>MVALQIPSLAATVRQDFPILNQEINGHPLVYLDNAATSQKPRAVLEKLMHYYENDNANVHRGAHQLSVRATDA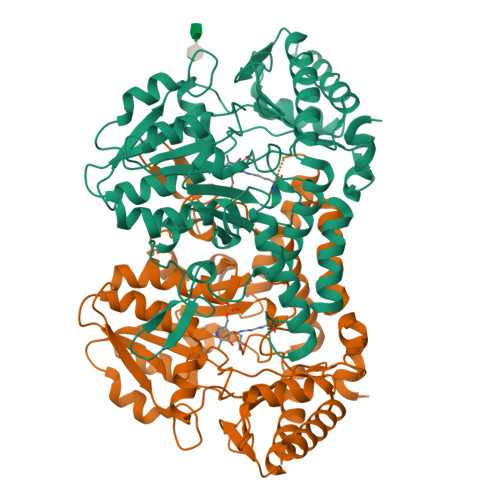YEAVRNKVAKFINARSPREIVYTRNATEAINLVAYSWGMNNLKAGDEIITTVMEHHSNLVPWQMVAAKTGAVLKFVQLDEQESFDLEHFKTLLSEKTKLVTVVHISNTLGCVNPAEEIAQLAHQAGAKVLVDACQSAPHYPLDVQLIDCDWLVASGHKMCAPTGIGFLYGKEEILEAMPPFFGGGEMIAEVFFDHFTTGELPHKFEAGTPAIAEAIALGAAVDYLTDLGMENIHNYEVELTHYLWQGLGQIPQLRLYGPNPKHGDRAALASFNVAGLHASDVATMVDQDGIAIRSGHHCTQPLHRLFDASGSARASLYFYNTKEEIDLFLQSLQATIRFFSDDDFTV[2x]> SGRGXG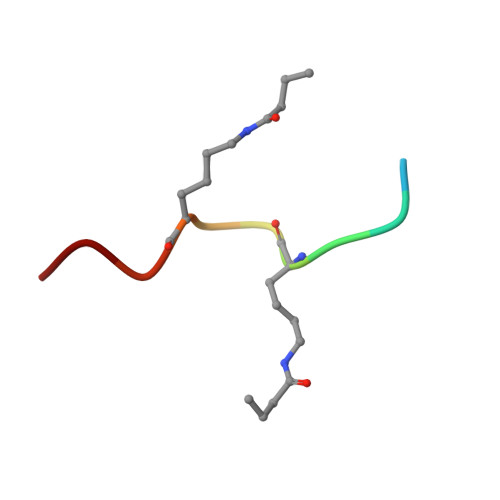GXGLG> MRQWTAIHLAKLARKASRAVGKRGTDLPGQIARKVDTDVLRKLAEQVDDIVFISGTNGKTTTSNLIGHTLKANNIQIIHNNEG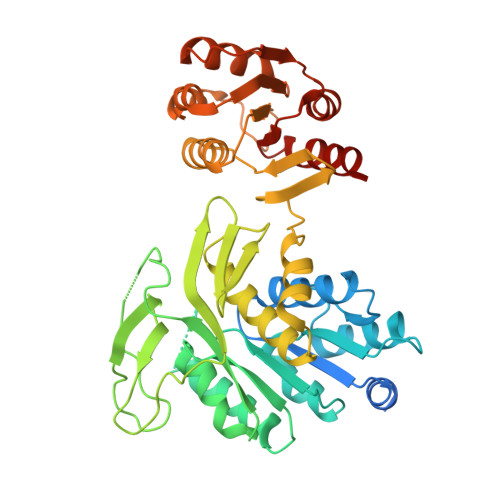ANMAAGITSAFIMQSTPKTKIAVIEIDEGSIPRVLKEVTPSMMVFTNFFRDQMDRFGEIDIMVNNIAETISNKGIKLLLNADDPFVSRLKIASDTIVYYGMKAHAHEFEQSTMNESRYCPNCGRLLQYDYIHYNQIGHYHCQCGFKREQAKYEISSFDVAPFLYLNINDEKYDMKIAGDFNAYNALAAYTVLRELGLNEQTIKNGFETYTSDNGRMQYFKKERKEAMINLAKNPAGMNASLSVGEQLEGEKVYVISLNDNAADGRDTSWIYDADFEKLSKQQIEAIIVTGTRAEELQLRLKLAEVEVPIIVERDIYKATAKTMDYKGFTVAIPNYTSLAPMLEQLNRSFEGGQS PIPERIDINE-3,4-DIOL | C5 H11 N O2 | 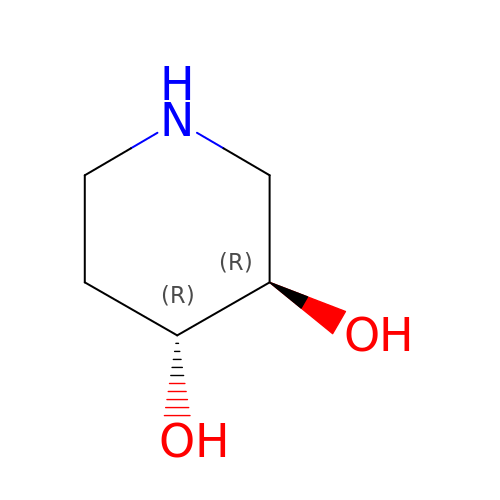IZXWMVPZODQBRB-RFZPGFLSSA-N>GVQPLATQCFQLSNMFNPQTEEEVGWDTEIKDDVIEECNKHGGVIHIYVDKYSAQGNVYVKCPSIAAAIAAVNALHGRWFAGKMITAAYVPLPTYHNLFPDSMTATQLLVPSRR[9x];>G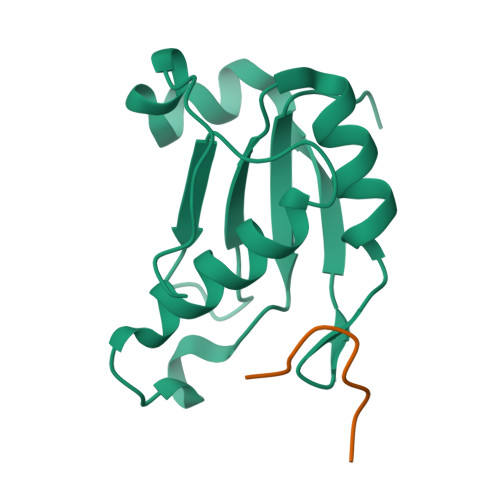KKKVRKYWDVPPPGFEHITPMQYKAMQA[9x]> MADKLRN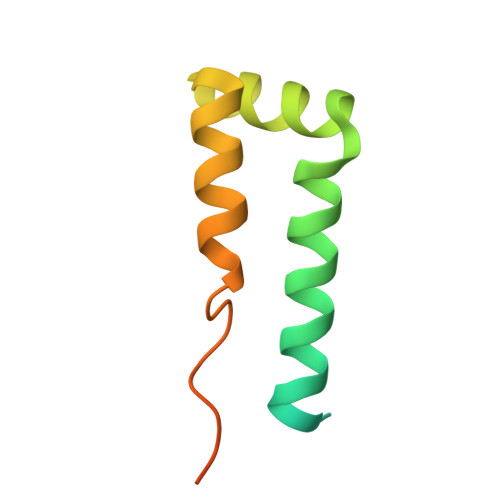QQELERLQAKYVGTGHPDTTSWEWKTNIHRDTYSSIVGHPPLLSYMALAQNEPVAKFRVQMIRKMLQPVGPPPPREEDIIMSNTQNGS methyl 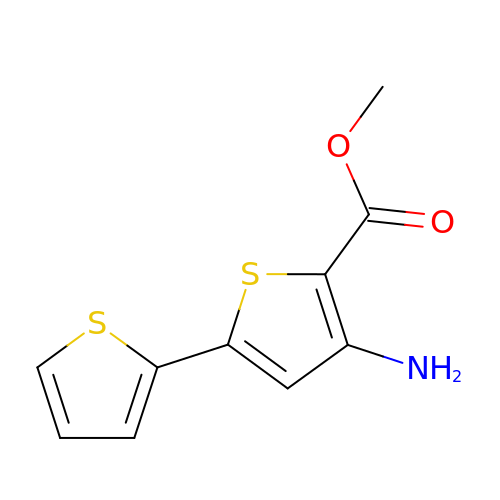3-azanyl-5-thiophen-2-yl-thiophene-2-carboxylate | C10 H9 N O2 S2 | CFHYAXQWEYGRTM-UHFFFAOYSA-N>GSHMGIKNDLEIRLQKLQQQGNFKNYLEQYPTDASTAAYFLIEIYNDGNIGGRSVIDAGTGNGILACGSYLLGAESVTAFDIDPDAIETAKRNCGGVNFMVADVSEISGKYDTWIMNPPFGSVVKHSDRAFIDKAFETSMWIYSIGNAKARDFLRREFSARGDVFREEKVYITVPRIYRHHSY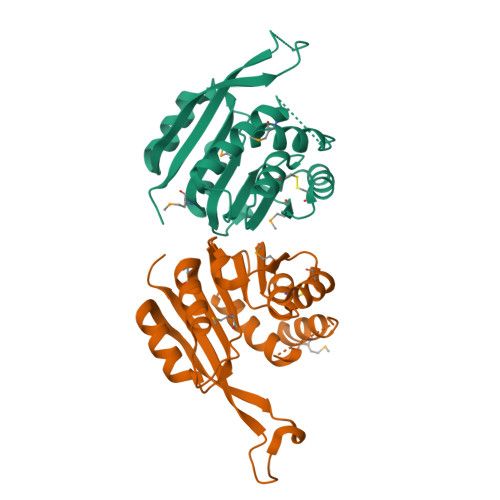DRARIEAVIFGVRNHSF[2x]> MKMLEQLEKKLGYTFKDKSLLEKALTHVSYSKKEHYETLEFLGDALVNFFIVDLLVQYSPNKREGFLSPLKAYLISEEFFNLLA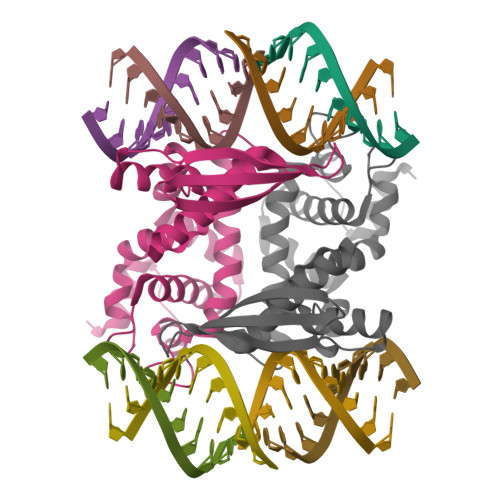QKLELHKFIRIKRGKINETIIGDVFKALWAAVYIDSGRDANFTRELFYKLFKEDILSAIKEGRVKKDYKTILQEITQKRWKERPEYRLISVEGPHHKKKFIVEAKIKEYRTLGEGKSKKEAEQRAAEELIKLLEES(2-methyl-3-phenyl-phenyl)methyl 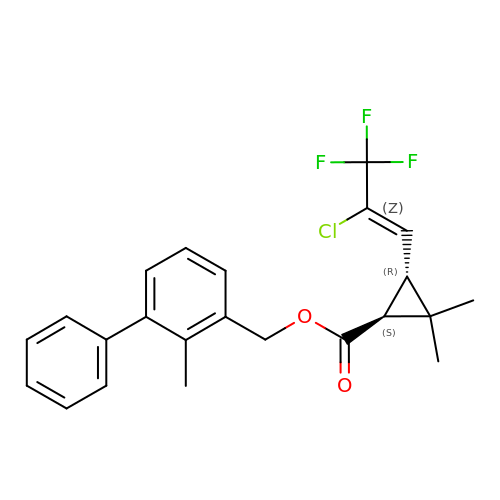(1~{S})-3-[(~{E})-2-chloranyl-3,3,3-tris(fluoranyl)prop-1-enyl]-2,2-dimethyl-cyclopropane-1-carboxylate | C23 H22 Cl F3 O2 | OMFRMAHOUUJSGP-AZUAARDMSA-N>[3x]ADDEDCCSYEDRREIRHIWDDVWSSSFTDRRVAIVRAVFDDLFKHYPTSKALFERVKIDEPESGEFKSHLVRVANGLKLLINLLDDTLVLQSHLGHLADQHIQRKGVTKEYFRGIGEAFARVLPQVLSCFNVDAWNRCFHRLVARIAKDLP;>[3x]KKQCGVLEGLKVKSEWGRAYGSGHDREAFSQAIWRATFAQVPESRSLFKRVHGDDTSHPAFIAHADRVLGGLDIAISTLDQPATLKEELDHLQVQHEGRKIPDNYFDAFKTAILHVVAAQLGRCYDREAWDACIDHIEDGIKGHH;>[3x]DEHEHCCSEEDHRIVQKQWDILWRDTESSKIKIGFGRLLLTKLAKDIPEVNDLFKRVDIEHAEGPKFSAHALRILNGLD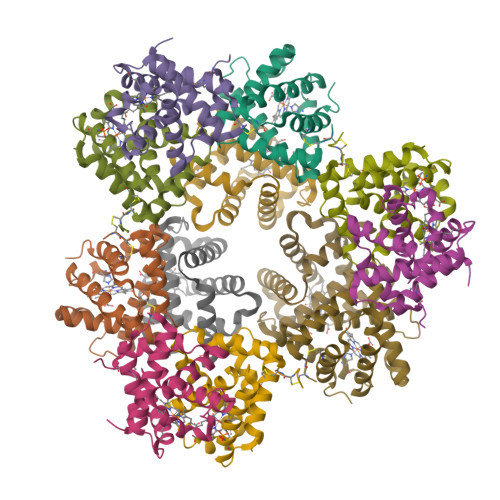LAINLLDDPPALDAALDHLAHQHEVREGVQKAHFKKFGEILATGLPQVLDDYDALAWKSCLKGILTKISSRLNA;>ECLVTESLKVKLQWASAFGHAHERVAFGLELWRDIIDDHPEIKAPFSRVRGDNIYSPEFGAHSQRVLSGLDITISMLDTPDMLAAQLAHLKVQHVERNLKPEFFDIFLKHLLHVLGDRLGTHFDFGAWHDCVDQIIDGIK[3x]> MPELFIMY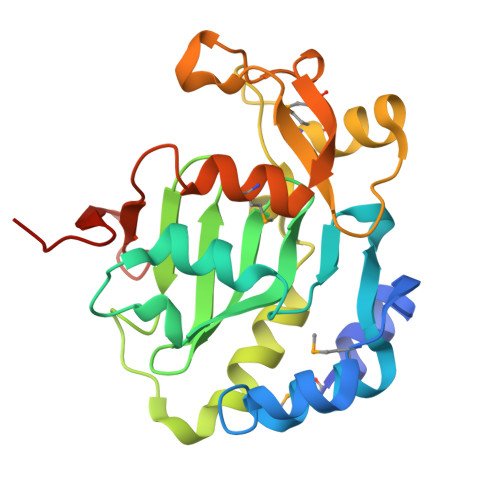ENALKRFGLPENPEIMGEADIARYKNRIPETYLDFIRHAGLGIWKQGYFQFCNPEKYKSIVALALGGDKQLNPVRTHALGFSAFGKILAWNEDYKTTEINILLHRVTCRGLFKEIPAERSDINLGIAVEGIDAESFDAPDEKGKLMFNRLLKNLGKLQLGQIYSPKLHPSLGGQLTVENMRPVDALSAMTIAAQAGPFTLYDTTKPSTPAVRTIGSLEHHHHHH>AEEFPVPNGFESAYREVDGVKLHYVKGGQGPLVMLVHGFGQTWYEWHQLMPELAKRFTVIAPDLPGLGQSEPPKTGYSGEQVAVYLHKLARQFSPDRPFDLVAHDIGIWNTYPMVVKNQADIARLVYMEAPIPDARIYRFPAFTAQGESLVWHFSFFAADDRLAETLIAGKERFFLEHFIKSHASNTE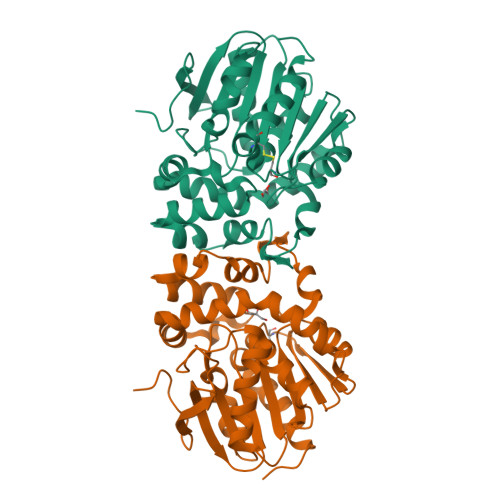VFSERLLDLYARSYAKPHSLNASFEYFRALNESVRQNAELAKTRLQMPTMTLAGGGHGGMGTFQLEQMKAYAEDVEGHVLPGCGHWLPEECAAPMNRLVIDFLSRGRHHHHHH[4x]>MSTNEGSLWGGRFAGGPSDALAALSKSTHFDWVLAPYDLTASRAHTMVLFRAGLLTEEQRDGLLAGLDSLAQDVADGSFGPLVTDEDVHAALERGLIDRVGPDLGGRLRAGRSRNDQVAALFRMWLRDAVRRVATGVLDVVGALAEQAAAHPSAIMPGKTHLQSAQPILLAHHLLAHAHPLLRDLDRIVDFDKRAAVSPYGSGALAGSSLGLDPDAIAADLGFSAAADNSVDATAARDFAAEAAFVFAMIAVDLSRLAEDIIVWSSTEFGYVTLHDSWSTGSSIMPQKKNPDIAELARGKSGRLIGNLAGLLATLKAQPLAYNRDLQEDKEPVFDSVAQLELLLPAMAGLVASLTFNVQRMAELA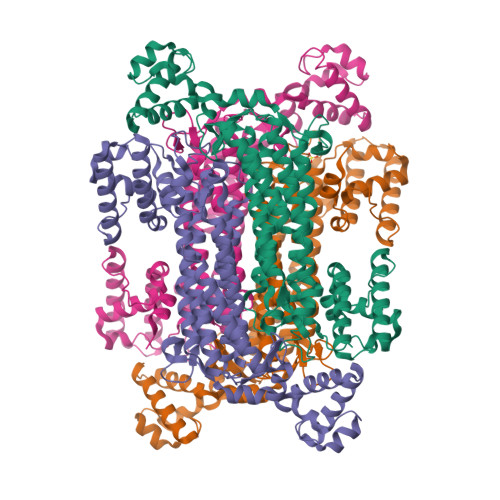PAGYTLATDLAEWLVRQGVPFRSAHEAAGAAVRAAEQRGVGLQELTDDELAAISPELTPQVREVLTIEGSVSARDCRGGTAPGRVAEQLNAIGEAAERLRRQLVR[4x]>AMHPRKDWYELTRATNWTPSYVTEEQLFPERMSGHMGIPLEKWESYDEPYKTSYPEYVSIQREKDAGAYSVKAALERAKIYENSDPGWISTLKSHYGAIAVGEYAAVTGEGRMARFSKAPGNRNMATFGMMDELRHGQLQLFFPHEYCKKDRQFDWAWRAYHSNEWAAIAAKHFFDDIITGRDAISVAIMLTFSFETGFTNMQFLGLAADAAEAGDYTFANLISSIQTDESRHAQQGGPALQLLIENGKREEAQKKVDMAIWRAWRLFAVLTGPVMDYYTPLEDRSQSFKEFMYEWIIGQFERSLIDLGLDKPWYWDLFLKDIDELHHSYHMGVWYWRTTAWWNPAAGVTPEERDWLEEKYPGWNKRWGRCWDVITENVLNDRMDLVSPETLPSVCNMSQIPLVGVPGDDWNIEVFSLEHNGRLYHFGSEVDRWVFQQDPVQYQNHMNIVDRFLAGQIQPMTLEGALKYMGFQSIEEMGKDAHDFAWADKCK[2x];>[2x]SFESKKPMRTWSHLAEMRKKPSEYDIVSRKLHYSTNNPDSPWELSPDSPMNLWYKQYRNASPLKHDNWDAFTDPDQLVYRTYNLMQDGQESYVQSLFDQFNEREHDQMVREGWEHTMARCYSPLRYLFHCLQMSSAYVQQMAPASTISNCC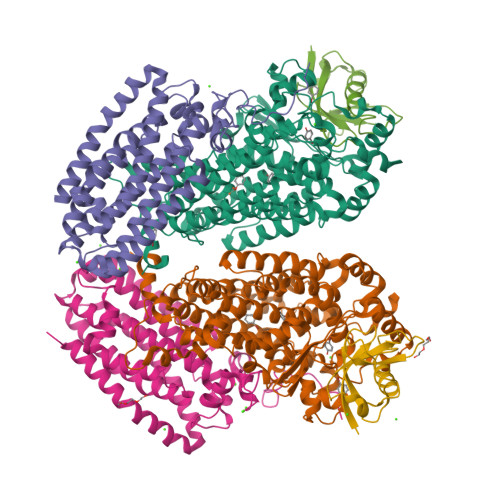ILQTADSLRWLTHTAYRTHELSLTYPDAGLGEHERELWEKEPGWQGLRELMEKQLTAFDWGEAFVSLNLVVKPMIVESIFKPLQQQAWENNDTLLPLLIDSQLKDAERHSRWSKALVKHALENPDNHAVIEGWIEKWRPLADRAAEAYLSMLSSD;>[2x]SAFPVHAAFEKDFLVQLVVVDLNDSMDQVAEKVAYHCVNRRVAPREGVMRVRKHRSTELFPRDMTIAESGLNPTEVIDVVFEE>AMADIGSEMKEYDVFIIGSGMAGMTIANKCASKGLTVGITDELPYGGTCALRGCDPKKVIIGATEVRDFAKRLKGSGIDTIPKVNWKDIMAFKQSFVDEMPPKVEKGYKRNGIDTFHSSAKFLSQNTLEIGNEKIKAKKIVIASGSKPRVLEFEGGHFAKTSADFLNLDELPKSLLFIGGGYIAFEFAHIAARCGAEVTIVHRGNNPLENFEQDIVKHLVSATKKLGVKLILNTDVTAIEKADKKFRVKGKSAEKTEYFEAEAVFNSAGRPPAIFDLELEKAGISFTKKGVSVNEHLQNTSNPIVYAAGDAADSEGLPLTPVAVLEGHTVASNIIKGNHKKISYPPMPTVVFTLPTMASVGYTESRARELNYNIQVNYKEVGDWFNAKRLNVAEYAFKTIIDEETQTILGAHLIGPHTEETINLFAMAIKTKMKVNDIRTMIFSYPTLASDIPHML[2x]

In this study, we identified and characterized mercuric reductase (GbsMerA), which is coded as a component of the mercury resistance (mer) operon in G. salicanalis isolated from Antarctic soil. We characterized GbsMerA, a mercury reductase belonging to the mercury-resistant operon of Gelidibacter salicanalis PAMC21136, and found its maximum activity of 474.7 µmol/min/mg in reducing Hg+2. As seen in the structures of thioredoxin reductase (high Mr), trypanothione reductase, glutathione reductase, glutathione amide reductase, and dihydrolipoamide dehydrogenase, the overall structure of GbsMerA also comprises an FAD-binding domain (residues 1–146), an NADPH-binding domain (residues 147–275), an interface domain (residues 276–340), and a dimerization domain (residues 341–447)29. GbsMerA has two pathways that connect molecular surfaces to the si- and re-faces of the isoalloxazine ring in FAD.

Crystals of GbsMerA (35 mg·mL−1) were obtained in drops of a 1:1 mixture of protein and crystallization buffer (1.6 M sodium phosphate monobasic/0.4 M potassium phosphate dibasic, 0.1 M sodium phosphate dibasic/citric acid [pH 4.2]). After interactive refinement of the coordinate, the structure was refined with a Rwork of 20.2% and a Rfree of 24.2% at 2.6Å. Two GbsMerA monomers, forming a homodimer with two-fold symmetry, were found in the asymmetric unit. Whole residues of the two monomers in the asymmetric unit could be built, except for regions 112–115 and 120–126 of chain B because of the unclear electron density. Non-covalently bound FAD is located in the central region of the FAD-binding domain, with two hydrophobic interactions, 16 hydrogen bonds, two water bridges, and π-stacking interactions. An unambiguous redox-active disulfide bond between Cys41 and Cys46 was found in the opposite NADPH-binding domain. In the si-face channel, two cysteines (Cys41 and Cys46) from the CXXXXC motif form a disulfide bond, and Asp47, Thr312, and Tyr437´ from the neighboring chain surround the disulfide bond and seem to be involved in the transfer of Hg2+ or the reduction of disulfide-bonded substrates. However, this His–Glu pair is substituted by Tyr437´ and Ser442´ in the corresponding region in the GbsMerA structure. The relative activity showed that Y437F completely lost its activity, indicating that the hydroxyl group of Tyr437 is important for metal coordination during transfer. Without NADPH, the side chain of Tyr174 points to the isoalloxazine ring of FAD by forming T-shaped configuration.> SMKLVKFRKGDSVGLRLAGGNDVGIFVAGVLEDSPAAKEGLEEGDQILRVNNVDFTNIIREEAVLFLLDLPKGEEVTILAQKKKDVYRRIVESDVGDSFYIRTHFEYEKESPYGLSFNKGEVFRVVDTLYNGKLGSWLAIRIGKNHKEVERGIIPNKNRAEQLASVQYTLPKTAGGDRADFWRFRGLRSSKRNLRKSREDLSAQPVQTKFPAYERVVLREAGFLRPVTIFGPIADVAREKLAREEPDIYQIAKSEPRDAGTDQRSSGIIRLHTIKQIIDQDKHALLDVTPNAVDRLNYAQWYPIVVFLNPDSKQ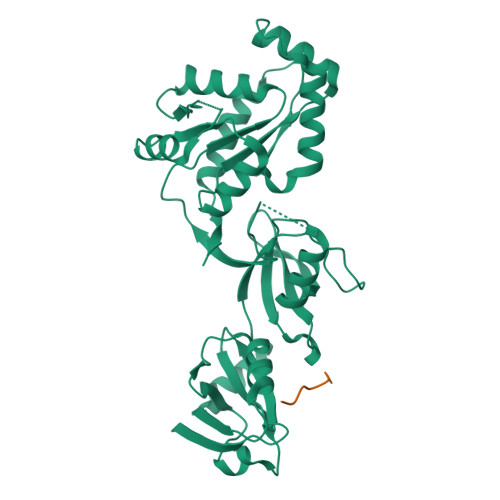GVKTMRMRLCPESRKSARKLYERSHKLRKNNHHLFTTTINLNSMNDGWYGALKEAIQQQQNQLVWVSEGKADGATSDDLDLHDDRLSYLSAPGSEYSMYSTDSRHTSDYEDTDTEGGAYTDQELDETLNDEVGTPPESAITRSSEPVREDSSGM;> SGDGKTSVWI> GSDDLVGVSVRPKVPLRTMSYKLAIDMSHFIKEKGGLEGIY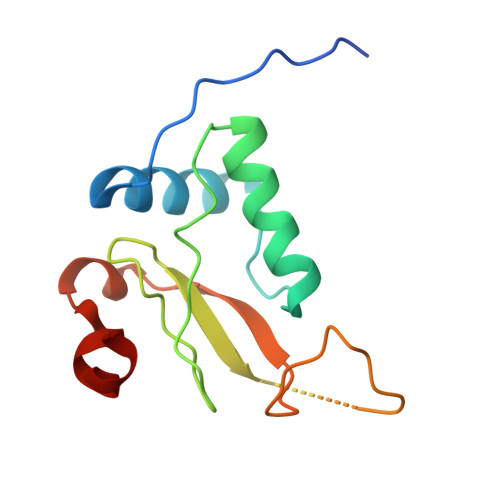YSARRHRILDIYLEKEEGIIPDWQDYTSGPGIRYPKTFGWLWKLVPVNVSDEAQEDEEHYLMHPAQTSQWDDPWGEVLAWKFDPTLAYTYEAYVRYPEEFGS>GAMGSKGAVVGIDLGTTNSCVAVMEGKQAKVLENAEGARTTPSVVAFTADGERLVGMPAKRQAVTNPNNTFYATKRLIGRRYDDPEVQKDIKNVPFKIVRASNGDAWVEAHGKLYSPSQIGAFVLMKMKETAENYLGHTAKNAVITVPAYFNDSQRQATKDAGQISGLNVLRVINEPTAAALAYGLDKSEDKVIAVYDLGGGTFDISILEIQKGVFEVKSTNGDTFLGGEDFDQALLRHIVKEFKRETGVDLTKDNMALQRVREAAEKAKCELSSSVQTDINLPYLTMDSSGPKHLNMKLTRAQFEGIVTDLIRRTIAPCQKAMQDAEVSKSDIGEVILVGGMTRMPKVQQTVQDLFGRAPSKAVNPDEAVAI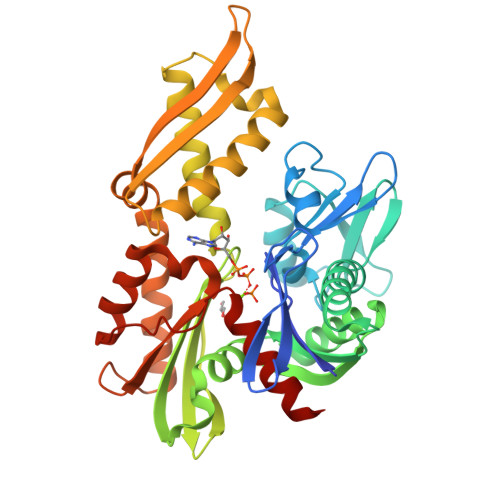GAAIQGGVLA[2x]> GLLGDDVEYAPLTVSVIVQDEGVDAIPVKVLNCDTISQVKEKIIDQVYRGQPCSCWPRPDSVVLEWRPGSTAQ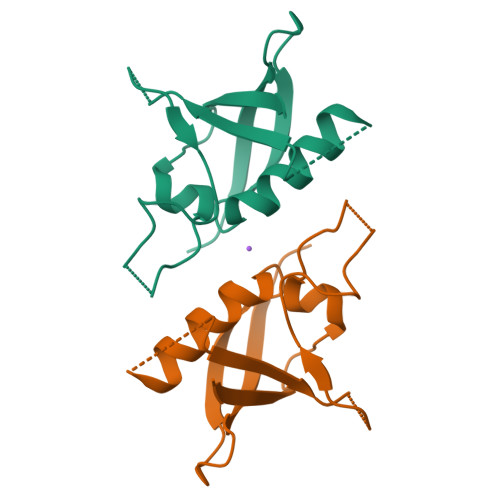ILSDLDLTSQREGRWKRVNTLMHYNVRDGATLILSKVG> TTEPTTSSSLCGIDHEALNKQIMEYKRRKDKGLG;> KLHIPVMVDEVVHCLSPQKGQIFLDMTFGSGGHTKAILQKESDIVLYALDRDPTAYALAEHLSELYPKQIRAMLGQFSQAEALLMKAGVQPGTFDGVLMDLGCSSMQLDTPERGFSLRKDGPLDMRMDGGRYPDMPTAADVVNALDQQALASILRTYGEEKHAKKIASAIVQARSIYPITRTQQLASIVAGAFPPSAIYTRKDLLQRSTHIATKTFQALRIFVNNELNELYTGLKTAQKFLRPGGRLVALSFHSLEDRIVKRFLLGISMTERFNLSVRQQVMKTSQLGSDHENTEEVSMRRAPLMWELIHKKVLSPQDQDVQDNPRGRSAKLRAAIKL

The m4C methyltransferase METTL15 maintains mitochondrial homeostasis by catalyzing m4C839 located in 12 S rRNA helix 44 (h44). Similar to other members of rRNA methyltransferases, METTL15 has a two-domain structure: an MTase domain (domain 1) and a scaffold-like domain (domain 2). The domain 2 of METTL15 contained five α-helices and one η-helix, which formed a scaffold for the binding of RNA substrates or other functional proteins. Here, we reported a series of crystal structures of human METTL15–hsRBFA–h44–SAM analog, METTL15–hsRBFA–SAM, METTL15–SAM and apo METTL15.

The METTL1570–407–RNA–hsRBFA226–260–SFG quaternary complex structure was subsequently refined to a resolution of 3.1 Å in space group C2221. In the structure of the quaternary complex, METTL15–RNA–hsRBFA226–260–SFG adopted a similar conformation to that in the METTL1570–407–hsRBFA226–260–SAM ternary complex, displaying an overall r.m.s.d. for Cα atoms of 0.475 Å. The helix of hsRBFA226–260 and the RNA substrate bound on either side of METTL15 domain2. Unexpectedly, both the 5’ end and the 3’ end of h44_dsRNA1 bases in the quaternary complex partially paired with the neighboring RNA in the next symmetry equivalent for better crystallization, respectively. Consistent with the previous FP assays, METTL15 interacted with the phosphodiester backbone of the RNA instead of the bases. The residues in the N-terminus of helix α7 and in the loop between helices α8 and α9 of METTL15 formed a positively charged channel to accommodate and recognize the RNA substrate. METTL15 His231, Lys234 and Arg270 formed several direct hydrogen bonds with the phosphodiester backbone of the RNA mainly via the positively charged side chain, while Phe262 and Pro263 recognized the phosphodiester backbone of the RNA via the hydrophobic interactions. The side chains of Pro263, Ala266 and Thr269 recognized the ribose of the RNA via the hydrophobic interactions. Strikingly, the alignment of our quaternary complex METTL1570–407–RNA–hsRBFA226–260–SFG structure with the RsmH structure showed that the helix of hsRBFA posed a physical barrier with the inactive cytidine in RsmH structure (indicated with a red circle).>MHHHHHHSQHKIFAKQDVRKLYLDEQGNVDFNKIQARWDELKNIKVSLANKHYTQAVVEKVKTMSAEDQQRFLDIVIAGLTNDDSQVGISATRPEDYDVFLFYLEPIIREYHKIEGETKQEHDWNIPVGEYVLTKIDPALEKVSMRARVARNVVGYNLPSSMDKDERIKFENQMVTVFENFGIPGNYYSLTPGHKNFISDQKADELRKRHFLFIDMTSDNHLMSNGVASDWPFGRGIWISQDESKMVWVGEEDQLRIISIVQGND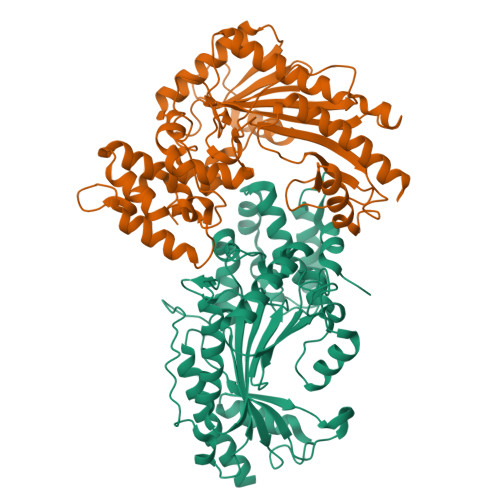LGKVDQSLHELLNGIEKSGLKFAEHPVYGIITTCPTNMGTGKRQSILGKFPNLSKAGTDEANLKDKAKSIGLQARGIGGEHSSVDQEGTADISPSARFGVTEAIVTKRLFEGLIVLYQIEKTTVPEKARNNCCTIF[2x]>GSTQEEIENLPAFPREKLTLRLLLGSGAFGEVYEGTAVDILGVGSGEIKVAVKTLKKGSTDQEKIEFLKEAHLMSKFNHPNILKQLGVCLLNEPQYIILELMEGGDLLTYLRKARMATFYGPLLTLVDLVDLCVDISKGCVYLERMHFIHRDLAARNCLVSVKDYTSPRIVKIGDFGLARDIYKNDYYRKRGEGLLP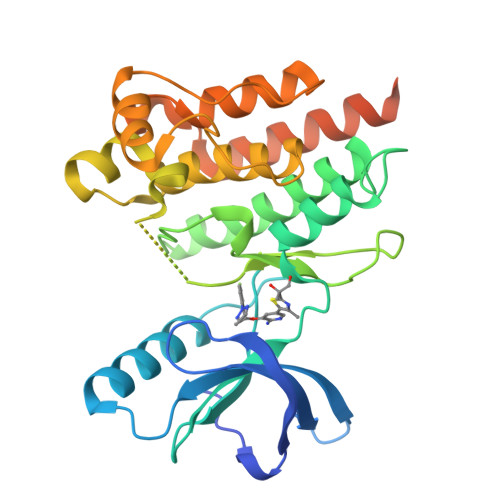VRWMAPESLMDGIFTTQSDVWSFGILIWEILTLGHQPYPAHSNLDVLNYVQTGGRLEPPRNCPDDLWNLMTQCWAQEPDQRPTFHRIQDQLQLFRNFFLNSIYKSRDEANNSGVINESFEGEDGDVICLNSDLE[2x]>[2x]MLPQRLHPSRLLALALFSLVLGLAGCQTKPPQTGLSAEQIA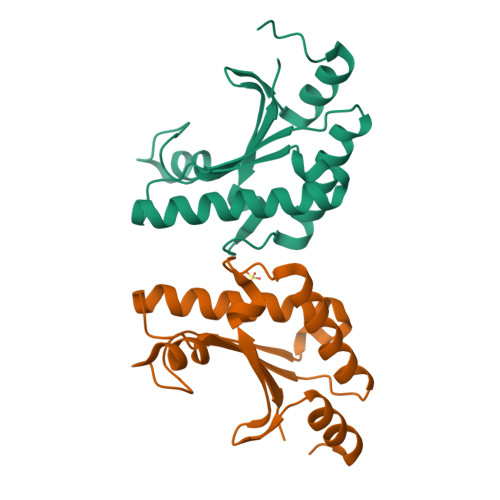VLQEQGFELRDEGWEFGMSSKVLFGNNLDRLNPDSRNTLTKIARALLAVDIDKVRLEGHTDNYGDEGYNQKLSERRAESVAAVFREAGMPAANIEVRGLGMSKPVADNKTRAGRSENRRVAIIVPAE> MSHHHHHHHHSENLYFQSGGGRDEIKERIFKAVVRAIVTGNP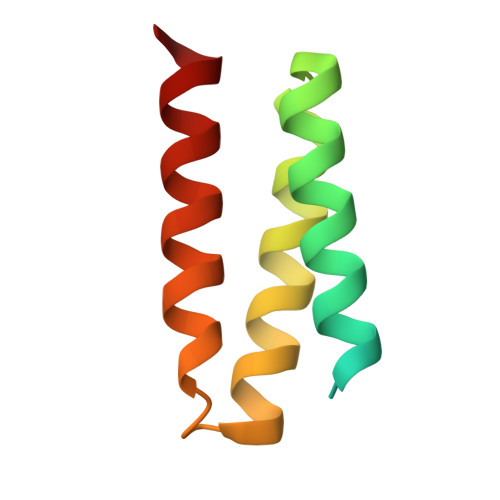EQLKEAKKLLEKLKKLGRLDQDAKKFEKAIRQVEKRLRS>MFERIDYYAGDPILGLVEKFAADNNPDKVNLGIGIYYDESGVMPVLDCVKIAEQRIADPISPRPYLPMAGLPGHRKGCQELLFGKDAPVLKDGLVATIATIGGSGALKVGAEFIHEWFPQSKCYVSDPTWGNHIAIFEGCDIEVGKYPYYDTATGGIKFDEMIAFFETLNKDDVLLLHPCCHNPTGVDLTREQWDTVLNVIQERELIPFMDIAYQGFGEDMDSDAYAIRKAVDMGLPLFVSNSFSKNLSLYGERVGGLSVVCPTVDETERVFGQLNSTVRRIYSSPPSHGGRVVDIVMNDAALHEQWVGEVYAMRD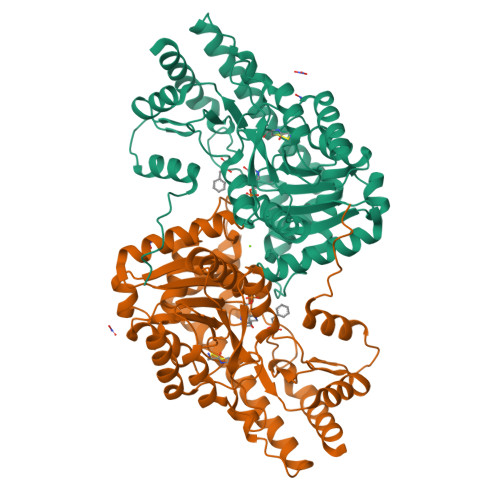RIKSMRTKLKSVLEAKISGRNFDYLTAQNGMFSFTGLTPEQVERLQSEFGIYMISNSRMCVAGLNSSNIDYVANAMVDVLKD[2x]2-[5-(1,3-benzodioxol-5-yl)-2-~{tert}-butyl-1~{H}-imidazol-4-yl]-6-methyl-pyridine | C20 H21 N3 O2 | 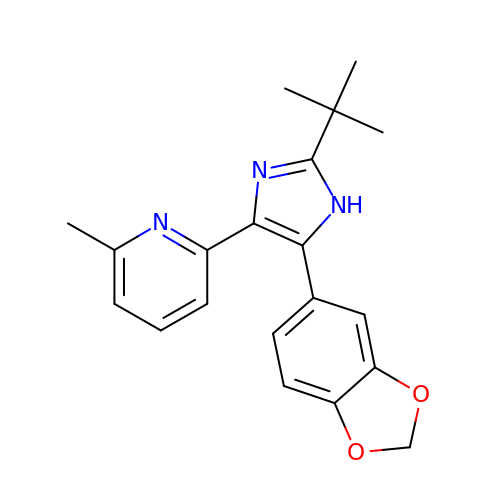WGZOTBUYUFBEPZ-UHFFFAOYSA-N> GASKIAALKEKIAALKEKIAALKEKIKDTELGMKELNEILIKEETVRRTLHNELQELRGNIRVYLRIRPALKNLENSDTSLINVNEFDDNSGVQSMEVTKIQNTAQVHEFKFDKIFDQQDTNVDVFKEVGQLVQSSLDGYNVAIFAYGQTGSGKTFTMLNPGDGIIPSTISHIFNWINKLKTKGWDYKVNAEFIEIYNENIVDLLRSDNNNKEDTSIGLKHEIRHDQETKTTTITNVTSVKLESEEMVEIILKKANKLRSTASTASNEHSSRSHSIFIIHLSGSNAKTGAHSYGTLNLVDLAGSERINVSQVVGDRLRETQNINKSLSALGDVIHALGQPDSTKRHIPFRNSKLTYLLQYSLTGDSKTLMFVNISPSSSHIN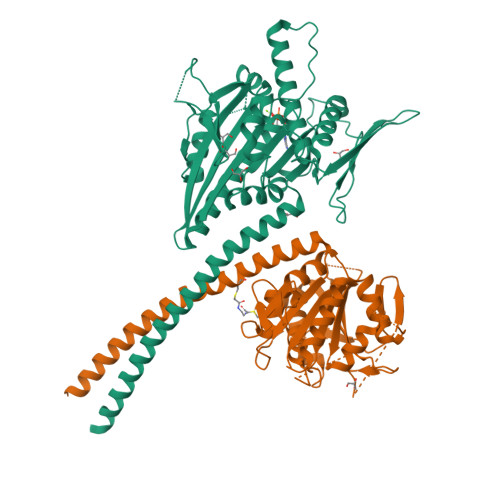ETLNSLRFASKVNSTRLVSRK;> GASEIAALEKEIAALEKEIAALEKEISKQEKFYNDTYNTVCKELLRSRRLENSIIEQKGTMRVYAYVMEQNLPENLLFDYENGVITQGLSEHVYKFNRVIPHLKVSEDCFFTQEYSVYHDMALNQKKNFNLISLSTTPHGSLRESLIKFLAEKDTIYQKQYVITLQFVFLSDDEFSQDMLLDYSHNDKDSIKLKFEKHSISLDSKLVIIENGLEDLPLNFSADEHPNLPHSGMGIIKVQFFPRDSKSDGNNDPVPVDFYFIELNNLKSIEQFDKSIFKKESAETPIALVLKKLISDTKSFFLLNLNDSKNVNKLLTISEEVQTQLAKRKKKLT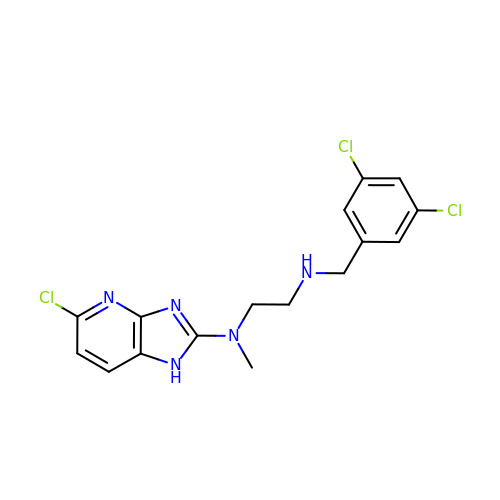5-chloro-N-(2-{[(3,5-dichlorophenyl)methyl]amino}ethyl)-N-methyl-3H-imidazo[4,5-b]pyridin-2-amine | C16 H16 Cl3 N5 | RQBUPIVTKWJGSG-UHFFFAOYSA-N>MGLNDNKAGMEGLDKEKINKIIMEATKGSRFYGNELKKEKQVNQRIENMMQQKAQITSQQLRKAQLQVDRFAMELEQSRNLSNTIVHIDMDAFYAAVEMRDNPELKDKPIAVGSMSMLSTSNYHARRFGVRAAMPGFIAKRLCPQLIIVPPNFDKYRAVSKEVKEILADYDPNFMAMSLDEAYLNITKHLEERQNWPEDKRRYFIKMGSSVENDNPGKEVNKLSEHERSISPLLFEESPSDVQPPGDPFQVNFEEQNNPQILQNSVVFGTSAQEVVKEIRFRIEQKTTLTASAGIAPNTMLAKVCSDKNKPNGQYQILPNRQAVMDFIKDLPIRKVSGIGKVTEKMLKALGIITCTELYQQRALLSLLFSETSWHYFLHISLGLGSTHLTRDGERKSMSVERTFSEINKAEEQYSLCQELCSELAQDLQKERLKGRTVTIKLKNVNFEVKTRASTVSSVVSTAEEIFAIAKELLKTEIDADFPHPLRLRLMGVRISSFPNEEDRKHQQ[2x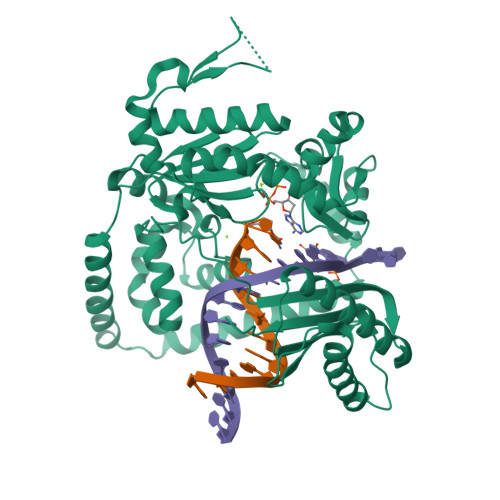]>[2x]GTSTQTKAGSLTIVGTGIESIGQMTLQALSYIEAAAKVFYCVIDPATEAFILTKNKNCVDLYQYYDNGKSRLNTYTQMSELMVREVRKGLDVVGVFYGHPGVFVNPSHRALAIAKSEGYRARMLPGVSAEDCLFADLCIDPSNPGCLTYEASDFLIRDRPVSIHSHLVLFQVGCVGIADFNFTGFDNNKFGVLVDRLEQEYGAEHPVVHYIAAMMPHQDPVTDKYTVAQLREPEIAKRVGG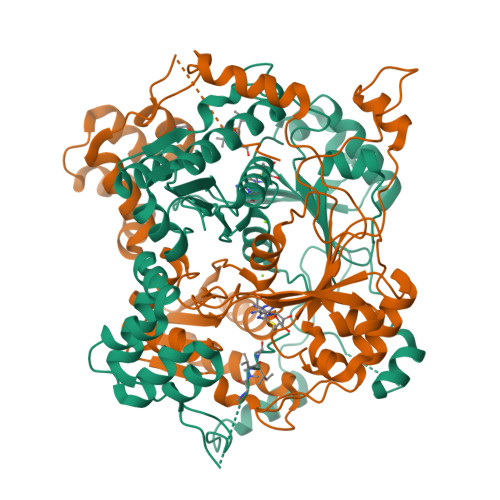VSTFYIPPKARKASNLDIIRRLELLPAGQVPDKKARIYPANQWEPDVPEVEPYRPSDQAAIAQLADHAPPEQYQPLATSKAMSDVMTKLALDPKALADYKADHRAFAQSVPDLTPQERAALELGDSWAIRCAMKNMPSSLLDAARESGEEASQNGFPWVIVVGVIGVIG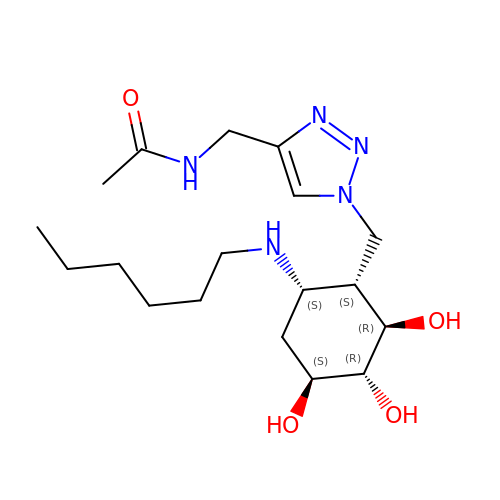~{N}-[[1-[[(1~{S},2~{R},3~{R},4~{S},6~{S})-6-(hexylamino)-2,3,4-tris(oxidanyl)cyclohexyl]methyl]-1,2,3-triazol-4-yl]methyl]ethanamide | C18 H33 N5 O4 | PGXKEXXUFBMCHO-NNPSNHGLSA-N>KKNGYPLDRNGKTTECSGVNAIAPHYCNSECTKVYYAESGYCCWGACYCFGLEDDKPIGPMKDITKKYCDVQIIPSGSHHHHHH[4x]

β-Scorpion toxins are polypeptides of 60–76 residues stabilized by four disulfide bridges. They bind with nanomolar affinity to an extracellular receptor (site 4) of voltage-gated sodium channels. β-Toxins induce a hyperpolarizing shift of the voltage-dependence of activation via a voltage-sensor trapping mechanism, whereby toxin-mediated interactions stabilize a persistently-activated conformation of the channel domain II voltage sensor. The extensively-characterized Bj-xtrIT from Hottentotta judaica is a member of the ‘excitatory’ (inducing a spastic paralysis) anti-insect β-toxins and its structure was the first of this class to be solved by X-ray crystallography. The toxins display variability in length, sequence, folds and molecular targets but share a common structural property in that in each case a network of disulfide bridges stabilizes their respective fold. This extensive reticulation establishes the tertiary structure that presents the bioactive surface as well as conferring significant thermostability and resistance to proteolysis.

In this study we show that the Bj-xtrIT β-scorpion toxin can be expressed in its natively-folded conformation by secretion of the polypeptide into the oxidizing environment of the E. coli periplasm. Instead, periplasmic co-secretion of the four bacterial chaperone proteins DsbC, DsbA, SurA and FkpA encoded by the pTUM4 plasmid enabled robust toxin over-expression. To produce natively-folded scorpion toxin directly from a bacterial expression system, we sub-cloned the Bj-xtrIT-(His6) gene into the pASK-IBA expression vector, thereby introducing an OmpA secretion signal at the toxin N-terminus. Purified Bj-xtrIT-(His6) toxin at a concentration of 10 mg/ml was mixed 1:1 (v/v) with 0.2 M NaCl, 0.1 M Bis-Tris; pH 5.5, 29% PEG 3350. Crystals of Bj-xtrIT-(His6) diffracted to 1.7 Å resolution and were solved by molecular replacement using the previously-reported Bj-xtrIT structure. Recombinant Bj-xtrIT-(His6) has both the βαββα-fold and C1–C4, C2–C6, C3–C7, and C5–C8 disulfide connectivity of the native fold. An all-atom structural superimposition of Bj-xtrIT-(His6) with the untagged Bj-xtrIT structure shows that there is a root-mean-square deviation (RMSD) of 0.45 Å. The structures differ only in side-chain rotamers for some residues located on the surface of the toxin, reflecting the difference in crystal contacts that the toxin forms under different crystal packing conditions (space groups C2221 vs I4122). Nevertheless the backbone atoms and disulfide groups all superimpose and show that recombinant Bj-xtrIT-(His6) was expressed with the native conformation. Localized denaturation of the α-helical regions could account for the temperature-dependent changes observed by SRCD signal, but overall the protein displayed significant thermostability that is consistent with a correctly-reticulated toxin structure.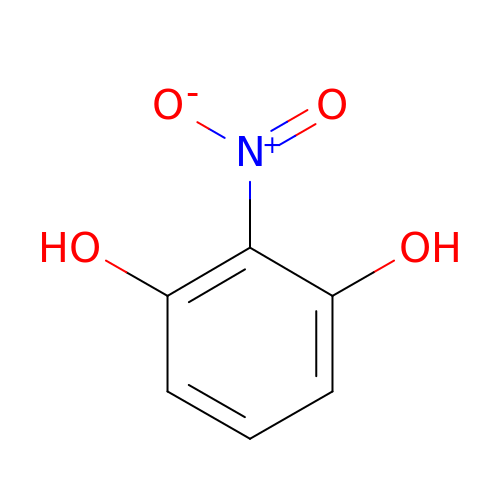2-nitrobenzene-1,3-diol | C6 H5 N O4 | ZLCPKMIJYMHZMJ-UHFFFAOYSA-N> MSTYEGRWKTVKVEIEDGIAFVILNRPEKRNAMSPTLNREMIDVLETLEQDPAAGVLVLTGAGEAWTAGMDLKEYFREVDAGPEILQEKIRREASQWQWKLLRMYAKPTIAMVNGWCFGGGFSPLVACDLAICADEATFGLSEINWGIPPGNLVSKAMADTVGHRQSLMYIMTGKTFGGQKAAEMGLVNESVPLAQLREVTIELARNLLEK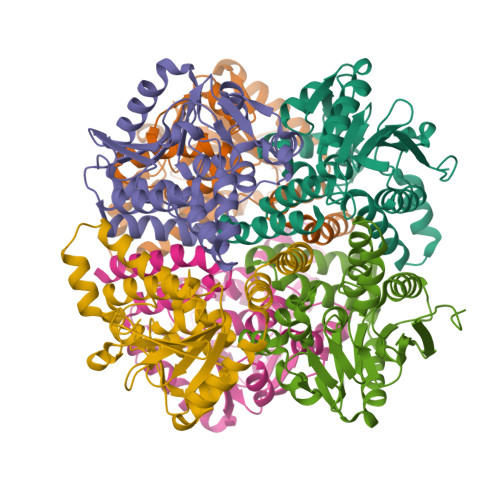NPVVLRAAKHGFKRCRELTWEQNEDYLYAKLDQSRLLDTEGGREQGMKQFLDDKSIKPGLQAYKR;>[10x]MSTYEGRWKTVKVEIEDGIAFVILNRPEKRNAMSPTLNREMIDVLETLEQDPAAGVLVLTGAGEAWTAGMDLKEYFREVDAGPEILQEKIRREASQWQWKLLRMYAKPTIAMVNGWCFGGGFSPLVACDLAICADEATFGLSEINWGIPPGNLVSKAMADTVGHRQSLYYIMTGKTFGGQKAAEMGLVNESVPLAQLREVTIELARNLLEKNPVVLRAAKHGFKRCRELTWEQNEDYLYAKLDQSRLLDTEGGREQGMKQFLDDKSIKPGLQAYKR;> MSTYEGRWKTVKVEIEDGIAFVILNRPEKRNAMSPTLNREMIDVLETLEQDPAAGVLVLTGAGEAWTAGMDLKEYFREVDAGPEILQEKIRREASQWQWKLLRMYAKPTIAMVNGWCFGGGFSPLVACDLAICADEATFGLSEINWGIPPGNLVSKAMADTVGHRQSLYYIMTGKTFGGQKAAEMGLVNESVPLAQLREVTIELARNLLEKNPVVLRAAKHGFKRCRELTWQQNEDYLYAKLDQSRLLDTEGGREQGMKQFLDDKSIKPGLQAYKR>[2x]MAETPNSDMSGATGGRSKRPKSNQDWWPSKLNLEILDQNARDVGPVEDDFDYAEEFQKLDLEAVKSDLEELMTSSQDWWPADYGHYGPLFIRMAWHSAGTYRTADGRGGAAGGRQRFAPINSWPDNANLDKARRLLLPIKQKYGQKISWADLMILAGNVAIESMGFKTFGYAGGREDAFEEDKAVNWGPEDEFETQERFDEPGEIQEGLGASVMGLIYVNPEGPDGNPDPEASAKNIRQTFDRMAMNDKETAALIAGGHTFGKVHGADDPEENLGPEPEAAPIEQQGLGWQNKNGNSKGGEMITSGIEGPWTQSPTEWDMGYINNLLDYEWEPEKGPG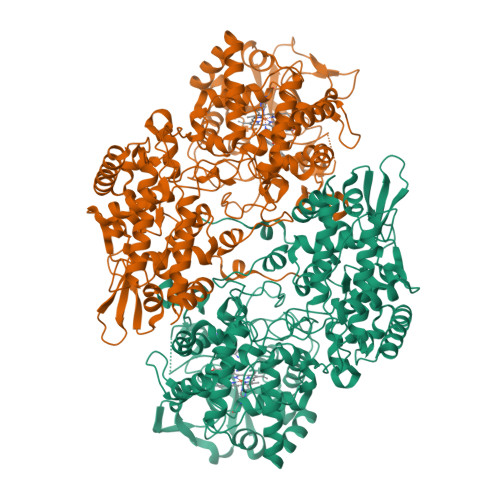GAWQWAPKSEELKNSVPDAHDPDEKQTPMMLTTDIALKRDPDYREVMETFQENPMEFGMNFAKAWYKLTHLDMGPPERFLGPEVPDEEMIWQDPLPDADYDLIGDEEIAELKEEILDSDLSVSQLVKTAWASASTYRDSDKRGGANGARLRLEPQKNWEVNEPEQLETVLGTLENIQTEFNDSRSDGTQVSLADLIVLGGNAAVEQAAANAGYDVEIPFEPGRVDAGPEHTDAPSFDALKPKVDGVRNYIQDDITRPAEEVLVDNADLLNLTASELTALIGGMRSIGANYQDTDLGVFTDEPETLTNDFFVNLLDMGTEWEPAADSEHRYKGLDRDTGEVKWEATRIDLIFGSNDRLRAISEVYGSADAEKKLVHDFVDTWSKVMKLDRFDLEHHHHHH>SNANFNRFTQRAKKAIDLAFESAKSLGHNIVGSEHILLGLLREEEGIAAKVLSKVGFTEAYLEGKIVDMEGKGEEISEDIVLSPRSKQILELSGMFANKLKTNYIGTEHILLAIIQEGEGIANKILNYA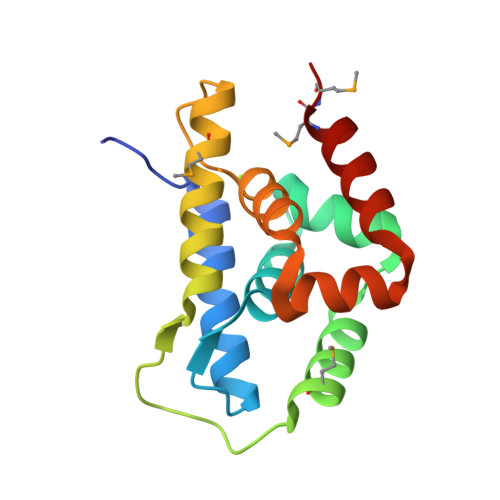GVNDRTLAQLTIDMMG[4x]>GSN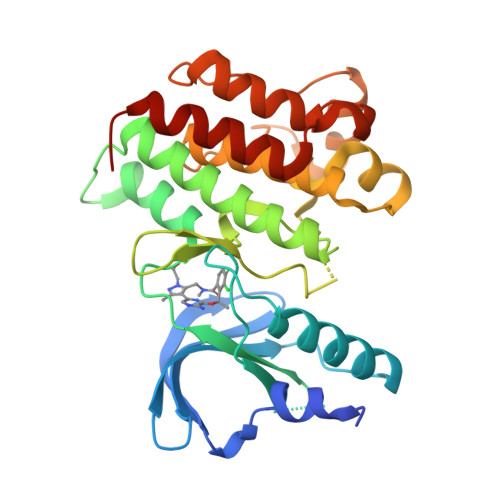SLGISEELKEKLRDVMVDRHKVALGKTLGEGEFGAVMEGQLNQDDSILKVAVKTMKIAICTRSELEDFLSEAVCMKEFDHPNVMRLIGVCFQGSERESFPAPVVILPFMKHGDLHSFLLYSRLGDQPVYLPTQMLVKFMADIASGMEYLSTKRFIHRDLAARNCMLNENMSVCVADFGLSKKIYNGDYYRQGRIAKMPVKWIAIESLADRVYTSKSDVWSFGVTMWEIATRGQTPYPGVENSEIYDYLRQGNRLKQPADCLDGLYALMSRCWELNPQDRPSFTELREDLENTLKALPPAQEPDE[4x]>[2x]MLNTTFANAKFANPFMNASGVHCMTIEDLEELKASQAGAYITKSSTLEKREGNPLPRYVDLELGSINSMGLPNLGFDYYLDYVLKNQKENAQEGPIFFSIAGMSAAENIAMLKKIQESDFSGITELNLSCPNVPGKPQLAYDFEATEKLLKEVFTFFTKPLGVKLPPYFDLVHFDIMAEILNQFPLTYVNSVNSI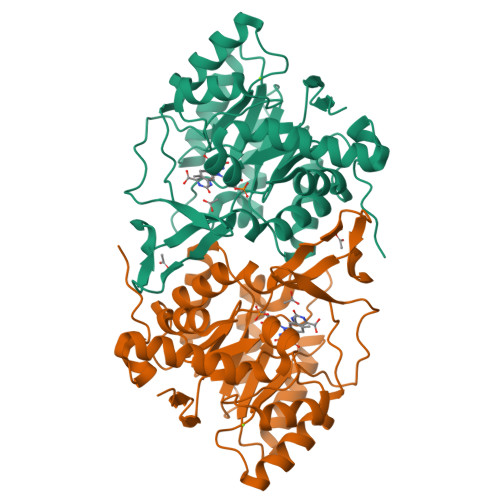GNGLFIDPEAESVVIKPEDGFGGIGGAYIKPTALANVRAFYTRLKPEIQIIGTGGIETGQDAFEHLLCGATMLQIGTALHKEGPAIFDRIIKELEEIMNQKGYQSIADFHGKLKSL dodecaethylene glycol monomethyl ether | C25 H52 O13 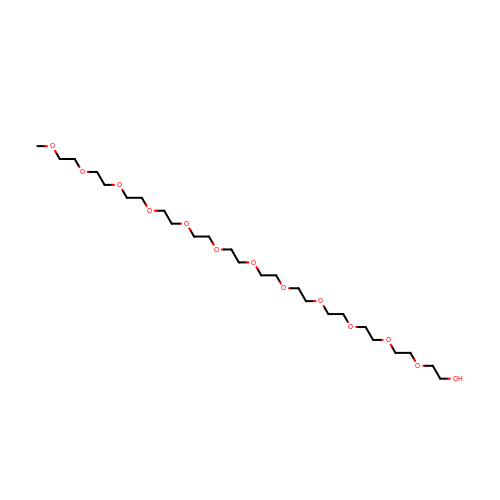| PLQZJIIDLZRWBG-UHFFFAOYSA-N>MAAPTPADKSMMAAVPEWTITNLKRVCNAGNTSCTWTFGVDTHLATATSCTYVVKANANASQASGGPVTCGPYTITSSWSGQFGP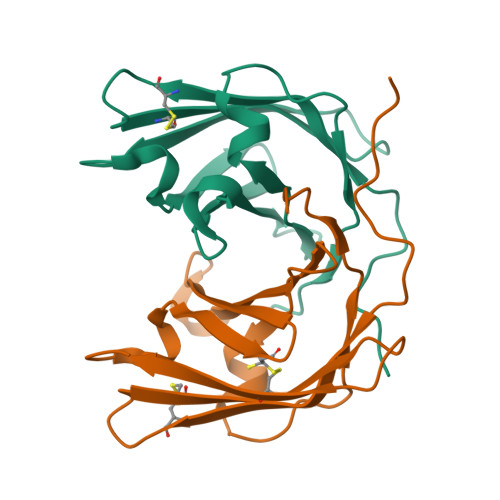NNGFTTFAVTDFSKKLIVWPAYTDVQVQAGKVVSPNQSYAPANLPLEHHHHHH[4x]> MGSDKIHHHHHHMDLKKLLPCG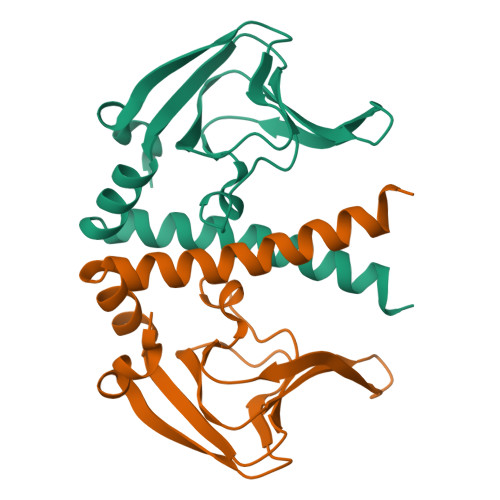KVIVFRKGEIVKHQDDPIEDVLILLEGTLKTEHVSENGKTLEIDEIKPVQIIASGFIFSSEPRFPVNVVAGENSKILSIPKEVFLDLLMKDRELLLFFLKDVSEHFRVVSEKLFFLTTKTLREKLMNFLVRHMNEKRELTLPVTLEELSRLFGCARPALSRVFQELEREGYIEKHGRRIKVLKNPFEHDRI>GAMVIEKEDVETNASNGQRVDLSSELDKLKKLENATVHMEFKPDAKAPAFYNLFSVSSATKKDEYFTMAVYNNTATLEGRGSDGKQFYNNYNDAPLKVKPGQWNSVTFTVEKPTAELPKGRVRLYVNGVLSRTSLRSGNFIKDMPDVTHVQIGATKRANNTVWGSNLQIRNL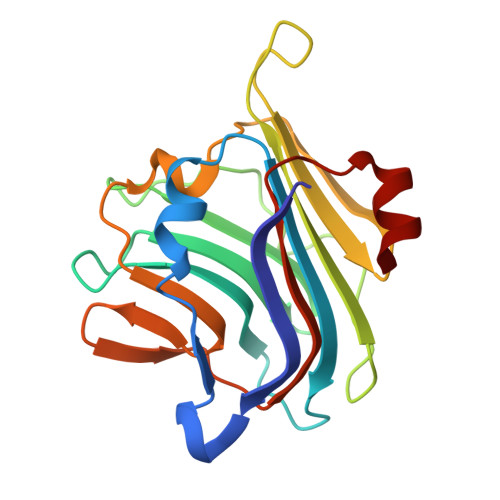TVYNRALTPEEVQKRS[2x]>KVPRGSHMLNVGATAPDFTLRDQNQQLVTLRGYRGAKNVLLVFFPLAFTGICQGELDQLRDHLPEFE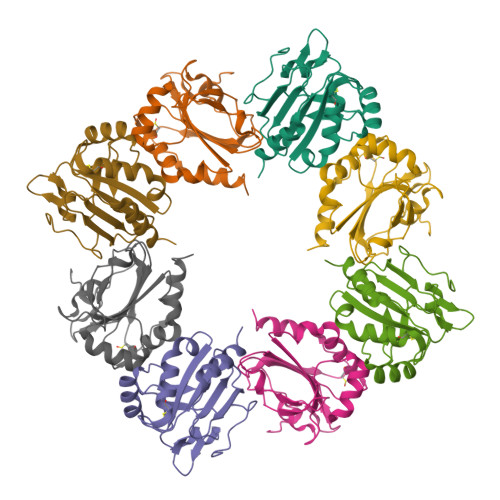NDDSAALAISVGPPPTHKIWATQSGFTFPLLSDFWPHGAVSQAYGVFNEQAGIANRGTFVVDRSGIIRFAEMKQPGEVRDQRLWTDALAALTA[2x]> SLTHRKFGGSGGSPFSGSGSGLSSIAVRSGSYLDAIIIDGVHHGGSGGNLSPTFTFGSGEYISNMTIRSGDYIDNISFETNMGRRFGPYG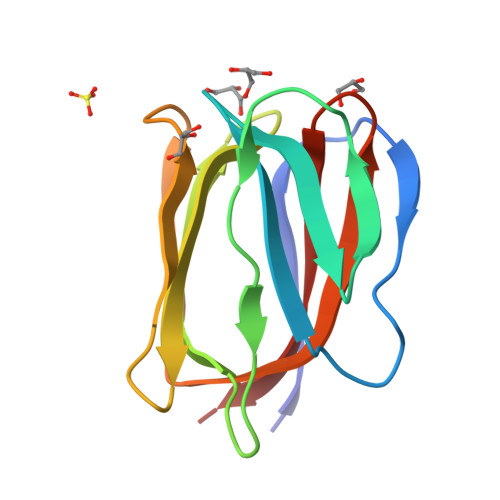GSGGSANTLSNVKVIQINGSAGDYLDSLDIYYEQY> GSHMVKKKEPAEGWPVVSGDYIVGDPESPVAAVTLASHIEDIPIDAGAAIAGPCKTENLGIEKVIANIISNPNIRFLVLCGSEVQGHIVGQSMKALHKNGVDD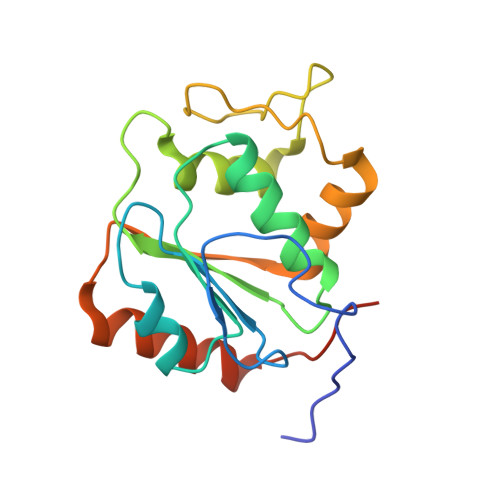KRKIIGAKGAIPYIENLPEEALERFQKQVEIVDLIDVEDADQIKEKVKECIEKDPGAFEEEEVILRL>MRRSFLKTIGLGVIALFLGLLNPLSAASYPPIKNTKVGLALSSHPLASEIGQKVLEEGGNAIDAAVAIGFALAVVHPAAGNIGGGGFAVIHLANGENVALDFREKAPLKATKNMFLDKQGNVVPKLSEDGYLAAGVPGTVAGMEAMLKKYGTKKLSQLIDPAIKLAENGYAISQRQAETLKEARERFLKYSSSKKYFFKKGHLDYQEGDLFVQKDLAKTLNQIKTLGAKGFYQGQVAELIEKDMKKNGGIITKEDLASYNVKWRKPVVGSYRGYKIISMSPPSSGGTHLIQILNVMENADLSALGYGASKNIHIAAEAMRQAYADRSVYMGDADFVSVPVDKLINKAYAKKIFDTIQPDTVTPSSQIKPGMGQLHEGSN[2x];>TTHYSVADRWGNAVSVTYTINASYGSAASIDGAGFLLNNEMDDFSIKPGNPNLYGLVGGDANAIEANKRPLSSMSPTIVLKNNKVFLVVGSPGGSRIITTVLQVISNVIDYNMNISEAVSAPRFHMQWLPDELRIEKFGMPADVKDNLTKMGYQIVTKPVMGDVNAIQVLPKTKGSVFYGSTDPRKEFGTGSKLAAAQLYTRASQPELAPEDPEDLEHHHHHHHH[2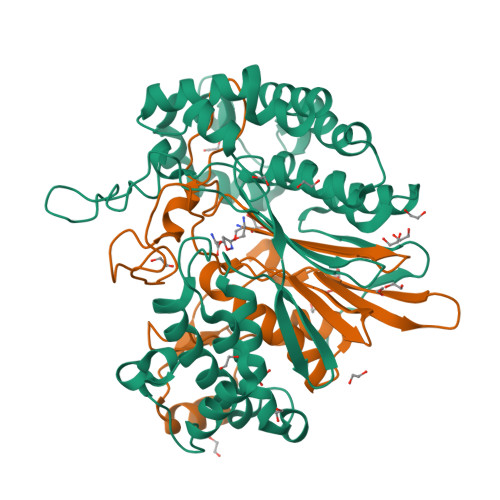x]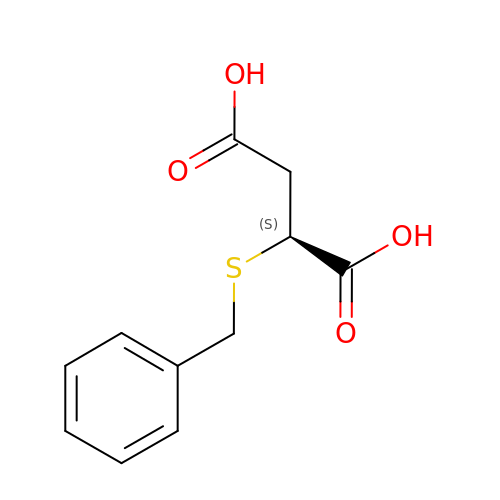(2~{S})-2-(phenylmethylsulfanyl)butanedioic acid | C11 H12 O4 S | PLQQDQFONINWJP-VIFPVBQESA-N Stimulator of interferon genes (STING) is an antiviral signalling protein that is broadly conserved in both innate immunity in animals and phage defence in prokaryotes. Here we use cryogenic electron microscopy to determine the structure of the active Toll/interleukin-1 receptor (TIR)–STING filament complex from a Sphingobacterium faecium cyclic-oligonucleotide-based antiphage signalling system (CBASS) defence operon. To define the molecular basis of STING filament formation, we reconstituted signalling of the S. faecium TIR–STING (SfSTING) antiphage effector in vitro and used single-particle cryo-EM to determine the structure of the activated complex. In each SfSTING dimer unit, the canonical V-shaped STING CBD is positioned above two TIR enzymatic NADase domains that dock against the base of the receptor.

In response to the nucleotide second messenger c-di-GMP produced during cyclic oligonucleotide-based antiphage signalling system (CBASS) immunity, SfSTING rapidly assembles into oligomers that form single filaments and antiparallel double-filament structures that make supra-molecular contacts between STING and TIR domains of opposing filaments. The TIR domains are not as well resolved in the main double-filament class, probably owing to conformational heterogeneity, and we therefore focused structural analysis on the single-fibre filaments. Additionally, a modest approximately 2° shift between packed SfSTING dimeric units is observed in both the single-fibre and wrapped double-fibre cryo-EM reconstructions, resulting in the active SfSTING filament structure adopting a slight curve.

>[12x]XXXXXXXXXXXXXXXXXXXXXXXXXXXXXXXXXXXXILIATKDDLTKQRGESLTKPRDNVVFEFGLFLGAAGPEKCYLIAEXXXXXXXXXXXXXXXXXXXEDTDLPTDLDGITVAKFTRNSGQYNSLDKIVESIRTHLVKIAEMSQLGLLPSTALAIGYYNSFIKRVCEEIHGSECVELEGKKIKVKSFRVDVVIPETLDDNGVGNFTTLYNKRYGLSKATTCTNPALLGTRGFPFHFKVDPPDANQESPVDIHLLDIPSTLSTIVESLKLYLPSNQVGQDFDMDYLEMRELENFAKVLKYLIGRNAATKGYVNVLTNVKL>[4x]MAHHHHHHMIREILKMGDPRLLRIADPVDHFDTPELHELVKDMFETMHDANGAGLAAPQIGVNLQ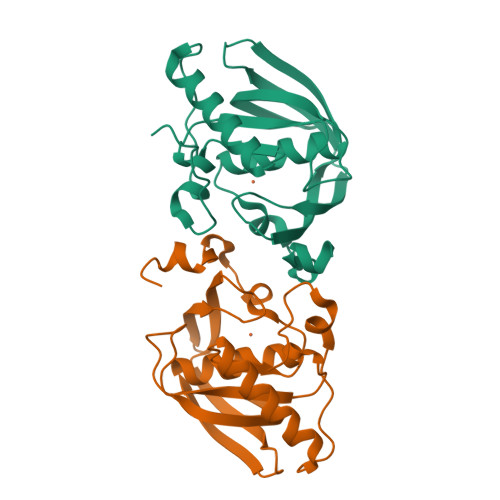VVIFGFGHNERYPDAPPVPETVLINPTITPVSQDMEEGWEGCLSVPGLRGAVSRFSMIKYHGFDQYGKPIDRVAEGFHARVVQHECDHLIGKLYPMRINDFAKFGFTEVLFPDMDPNSDD> MWGKKDAGTELTNYQTLATNTIGMMKGVDGYAFTSGAKMTDTLIQAGAAKGMTVSGDPASGSATLWNSWGGQIVVAPDTAGGTGFNNGFTITTNKVPQSACVSISTGMSRSGGTSGIK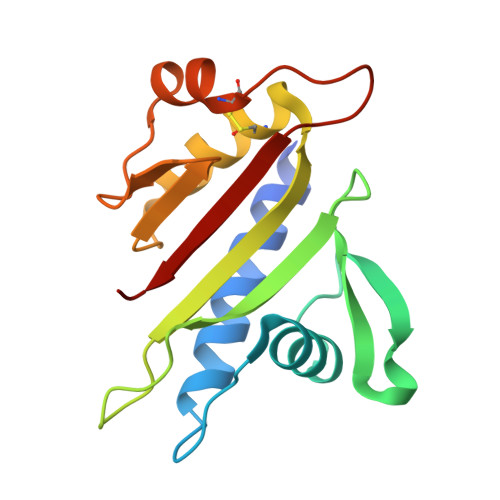INGNNHTDAKVTAEIASSECTADNGRTGTNTLVFNYNG> VVEQSKICSSHYEPTVRIGGRDGLCVDVSDNAYNNGNPIILWKCKDQLEVNQLWTLKSDKTIRSKGKCLTTYGYAPGNYVMIYDCSSAVAEATYWDIWDNGTIINPKSGLVLSAESSSMGGTLTVQKNDYRMRQGWRTGNDTSPFVTSIAGFFKLCMEAHGNSMWLDVCDITKEEQQWAVYPDGSIRPVQNTNNCLTCEEHKQGATIVMMGCSNAWASQRWVFKSDGTIYNLYDDMVMDVKSSDPSLKQIILWPYTGNANQMWA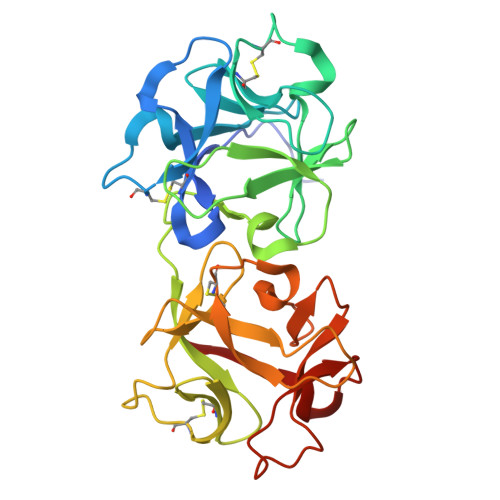TLF> QENQDGRYSLTYIYTGLSKHVEDVPAFQALGSLNDLQFFRYNSKDRKSQPMGLWRQVEGMEDWKQDSQLQKAREDIFMETLKDIVEYYNDSNGSHVLQGRFGCEIENNRSSGAFWKYYYDGK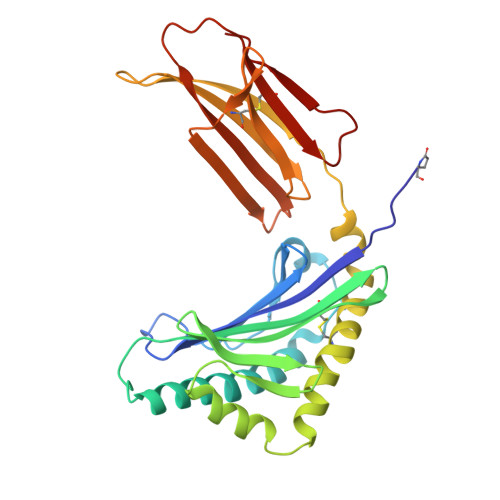DYIEFNKEIPAWVPFDPAAQITKQKWEAEPVYVQRAKAYLEEECPATLRKYLKYSKNILDRQDPPSVVVTSHQAPGEKKKLKCLAYDFYPGKIDVHWTRAGEVQEPELRGDVLHNGNGTYQSWVVVAVPPQDTAPYSCHVQHSSLAQPLVVPWEAS> XTIVALKYPGGVVMAGDRRSTQGNMISGRDVRKVYITDDYTATGIAGTAAVAVEFARLYAVELEHYEKLEGVPLTFAGKINRLAIMVRGNLAAAMQGLLALPLLAGYDIHASDPQSAGRIVSFDAAGGWNIEEEGYQAVGSGSLFA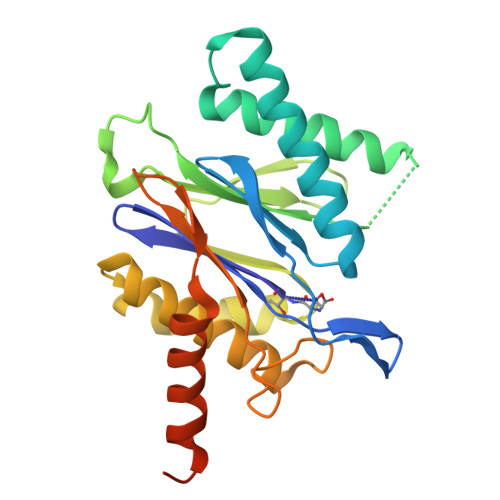KSSMKKLYSQVTDGDSGLRVAVEALYDAADDDSATGGPDLVRGIFPTAVIIDADGAVDVPESRIAELARAIIESRSGADTFGSDGGEKHHHHHH>[2x]MASMTGGQQMGRGSMHHHHMKYKITVETGDLRGAGTDASVSIKLTGKDGAETSAFSLDKYFHNDFESGGTDTYDQSGVDVGEIAMITLKE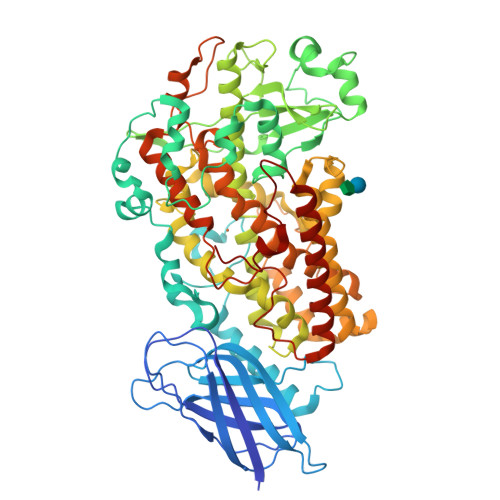NGFGLKSDWYIAKVIIEKIDEATGFSNKYIFPCYRWVIKQLVVYEGKAILPNSKDNVKTIAEQRTKEVSENKKLYKWGTDPRYVQDLPGFVDAEEPKSLPKDVQFTDEATSSLFRVGLADFANLGLSHLFGIWDDWDCLEDFRQLITPAIKSGLPHAAEYWRDDVWFGSQFLNGSNPEVIRRCDKLPENFPVKNEMVEKLLDRGYTLEKAMKEGLIFITDYKILEGIPTMDTPEDKRYITTPLGLFYLKNNDDIIPIAIQLYQQPGENNSIWTPLKDTEWDWIMAKLWLRCADTQYHQMITHLLRCHLMMEPTAVSSWRNLPSVHPVWKLLYPHTKGIMAINTLGRNDLIPTGGAADKVLSIGGGGQVTLMQKHYRSVTFDSYDLVKDLRQRGVDGLRKFYYKDDALLLWNVIHQFVQDIIQIYYNDDDSVKKDNEIQDWIRDLHENGYPAGSDGTDKKVPKSFENREELVHFLTVVVFTCSCQHAAVNFSQMATYGFHPNSPTLMRQPPPTEKGKSNHKVIMASLANKHQAVTMVSVVNALTTIYPTEKFLGDYADNLFGDAAAHAAMAKFKSNLANITKQITERNQGMVSPYTWLIPGHVPNSIAI5-[(3-aminopropyl)amino]pentane-1-thiol | C8 H20 N2 S | 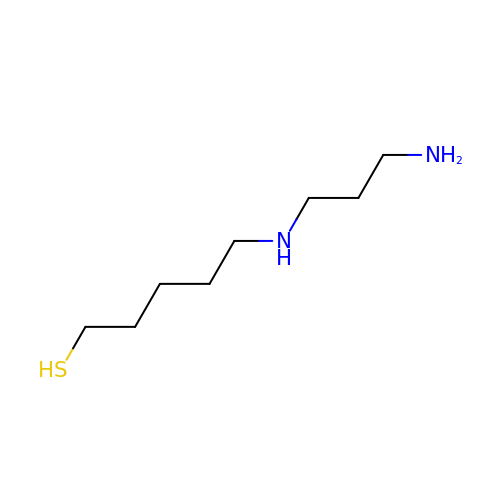UEAAWEWNMXIYCA-UHFFFAOYSA-N> MAISIKTPEDIEKMRVAGRLAAEVLEMIEPYVKPGVSTGELDRICNDYIVNEQHAVSACLGYHGYPKSVCISINEVVCHGIPDDAKLLKDGDIVNIDVTVIKDGFHGDTSKMFIVGKPTIM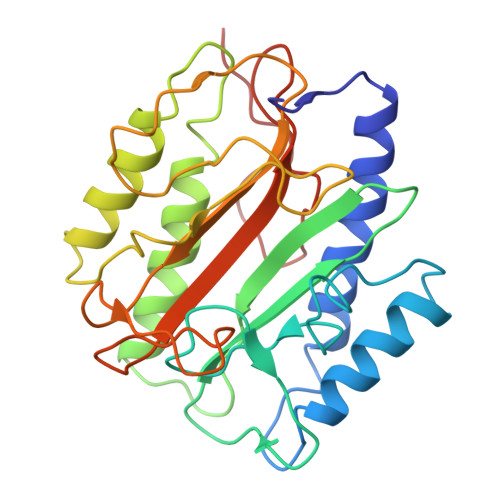GERLCRITQESLYLALRMVKPGINLREIGAAIQKFVEAEGFSVVREYCGHGIGQGFHEEPQVLHYDSRETNVVLKPGMTFTIEPMVNAGKKEIRTMKDGWTVKTKDRSLSAQYEHTIVVTDNGCEILTLRKDDTIPAIISHDE>QEERNQQQDDIEELETKAVGMSND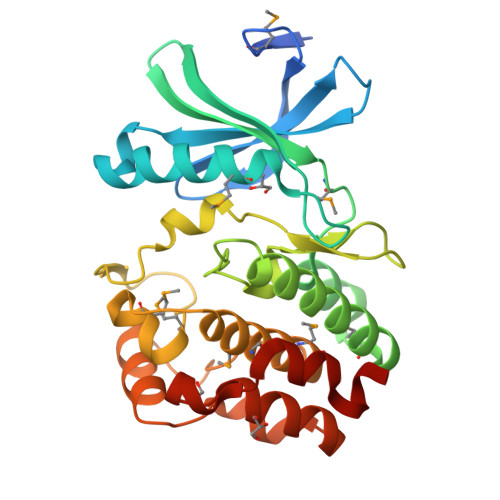GRFLKFDIEIGRGSFKTVYKGLDTETTVEVAWCELQDRKLTKSERQRFKEEAEMLKGLQHPNIVRFYDSWESTVKGKKCIVLVTELMTSGTLKTYLKRFKVMKIKVLRSWCRQILKGLQFLHTRTPPIIHRDLKCDNIFITGPTGSVKIGDLGLATLKRASFAKSVIGTPEFMAPEMYEEKYDESVDVYAFGMCMLEMATSEYPYSECQNAAQIYRRVTSGVKPASFDKVAIPEVKEIIEGCIRQNKDERYSIKDLLNHAFFQEET[2x]>[2x]MHHHHHHHMAQAAPAAAKAAAPSISRDEVEKCINAIRFLAIDAINKSKSGHPGMPMGCAPMGYVLWNEVMKYNPKNPDFFNRDRFVLSAGHGSMFQYSMMHLTGYDSVPLDQIKQFRQWNSLTPGHPENFVTPGVEVTTGPLGQGICNAVGLAVAEAHLAARFNKPDVKPIVDHYTYCILGDGCMMEGISNEACSLAGHWGLGKLIALYDDNKISIDGHTDISFTEDVAKRYEALGWHVIHVINGNTDVDGLRAAIAQAKAVKDKPTLIKVSTLIGYGSPNKADSHDVHGAPLGPDETAATRKNLNWPYGEFEVPQDVYDVFRGAIKRGAE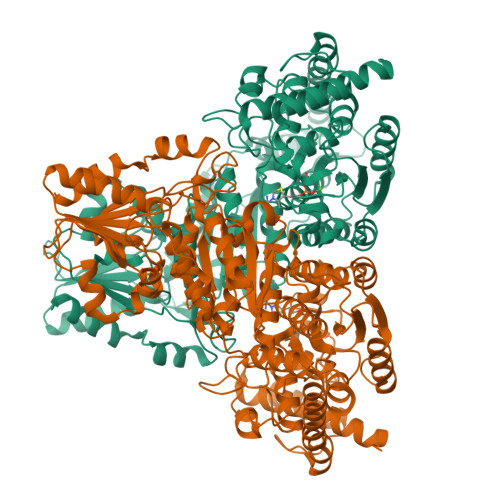EEANWHKACAEYKAKYPKEWAEFEALTSCKLPENWEAALPHFKPEDKGLATRQHSQTMINALAPALPGLIGGSADLAPSNLTLMKISGDFQKGSYAERNLRFGVREHAMGAICNGIALHKSGLIPYCATFYIFTDYMRNAMRMSALSEAGVVYVMTHDSIGLGEDGPTHQPIEHLASFRAMPDMLMIRPAGGNETAGAYKVAIANRKRPTTIALSRQNMPNIPNCSVEGVAKGAYTIHDTKAGVKPDVILMGTGSELELATAAAGILEKEGKNVRVVSFPCWELFEEQSAEYKESVLPSDVTARVSVEAATSFGWAKYIGLKGKHVGIDTFGASAPAPTLYEKFGITVNHVVEAAKATLQH> MSETRMAQNMDTTDEQYLRLIELLSNYDSTLEQLQKGFQDGYIQLSRSNYYNKDSLRGNYGEDYWDETYIGQLMATVEEKNSKVVVEIVKRKAQDKQEKKEEEDNKLTQRKKGTKPEKQKTQ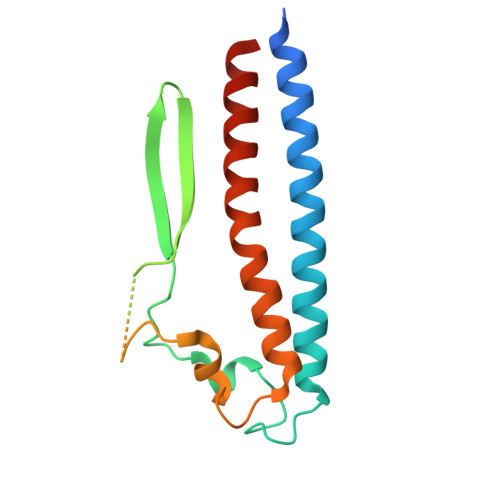SHKLKQDYDPILMFGGVLSVPSSLRQSQTSFKGCIPLIAQLINYKNEILTLVETLSEQE>MRIGEWMRGLLLCAGLMMCGVVHADISTVPDETYDALKLDRGKATPKETYEALVKRYKDPAHGAGKGTMGDYWEPIAISIYMDPNTFYKPPVSPKEVAERKDCVECHSDETPVWVRAWKRSTHANLDKIRNLKSDDPLYYKKGKLEEVENNLRSMGKLGEKETLKEVGCIDCHVDVNKKDKADHTKDIRMPTADTCGTCHLREFAERESERDTMVWPNGQWPAGRPSHALDYTANIETTVWAAMPQREVAEGCTMCHTNQNKCDNCHTRHEFSAAESRKPEACATCHSGVDHNNWEAYTMSKHGKLAEMNRDKWNWEVRLKDAFSKGGQNAPTCAACHMEYEGEYTHNITRKTRWANYPFVPGIAENITSDWSEARLDSWVLTCTQCHSERFARSYLDLMDKGTLEGLAKYQEANAIVHKMYEDGTLTGQKTNRPNPPEPEKPGFGIFTQLFWSKGNNPASLELKVLEMAENNLAKMHVGLAHVNPGGWTYTEGWGPMNRAYVEIQDEYTKMQELSALQARVNKLEGKQTSLLDLKGTGEKISLGGLGGGMLLAGALALIGWRKRKQTRA[6x];>MNKVIVAAFV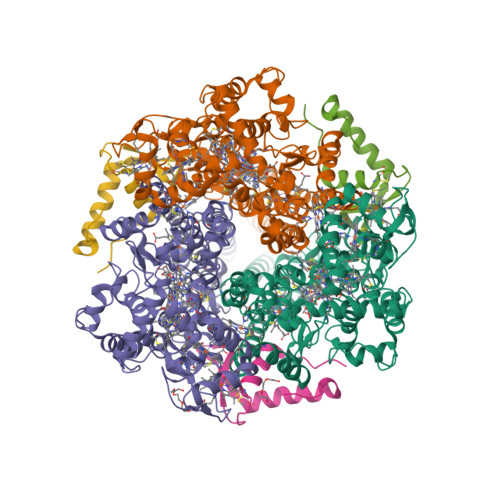SAFVLGSTATFASGNLESSLAPISAKDMLDYLACKDKKPTDVVKSHTEVENGKIVRVKCGDIVALVQKAREQSGDAWQGGY[6x]(1R,4R,5S,6S,7R,10R,11S,12S)-1,7-bis(hydroxymethyl)-2,8,13,14-tetraoxatricyclo[8.2.1.1~4,7~]tetradecane-5,6,11,12-tetrol 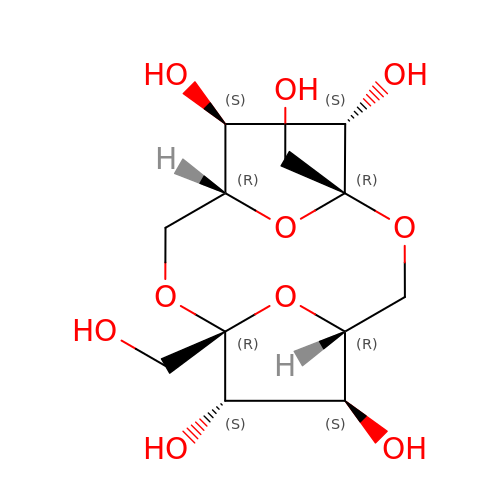| C12 H20 O10 | WMUHBTATSZQNJG-TWOHWVPZSA-N> GSKFSAKRLPSTRLGTFLENRVNDFLRRQNHPESGEVTVRVVHASDKTVEVKPGMKARFVDSGEMAESFPYRTKALFAFEEIDGVDLCFFGMHVQEYGSDCPPPNQRRVYISYLDSVHFFRPKCLRTAVYHEILIGYLEYVKKLGYTTGHIWACPPSEGDDYIFHCHPPDQKIPKPKRLQEWFKKMLDKAVSERIVHDYKDIFKQATEDRLTSAKELPYFEGDFWPNVLEESIKESGGSGSQKLYATMEKHKEVFFVIRLIAGPAANS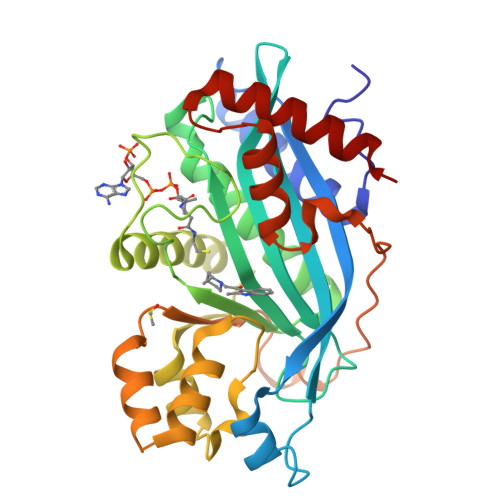LPPIVDPDPLIPCDLMDGRDAFLTLARDKHLEFSSLRRAQWSTMCMLVELHTQSQ>MDFKYTEEKETIKINNIMIHKYTVLYTSNCIMDIYSEEEKITCFSNRLVFLERGVNISVRMQKQILSEKPYVAFRLNGDMLRHLKDALMIIYGMSKIDTNACRSMSRKIMTTEVNKTLLDELKNINSHDNSAFISSLIYLISKLENNEKIIESIYISSVSFFSDKVRNLIEKDLSRKWTLGIIADAFNASEITIRKRLESENTNFNQILMQLRMSKAALLLLENSY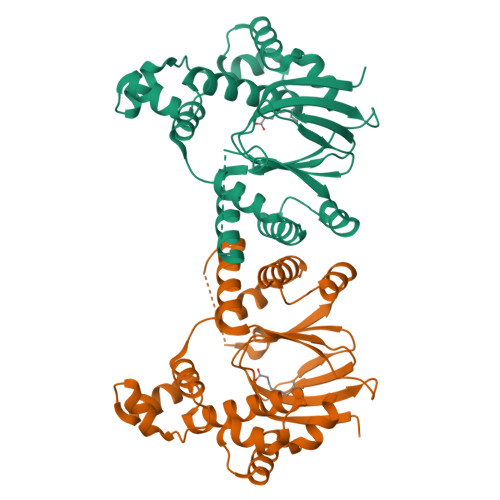QISQISNMIGISSASYFIRIFNKHYGVTPKQFFTYFKGG[2x]> GRGSEDFQYAIDMFKKFIEEAAASMGPEAVKYAKEFLKLLKEYHKNGINNRLLKIALLLLRNQKKIVDKASQDLWRRHPELIAPGGIAFSQRDRALCLRDYGWFLILIVMCLVSGDKGPIEKIGLKCIREMYNSLGVVPAM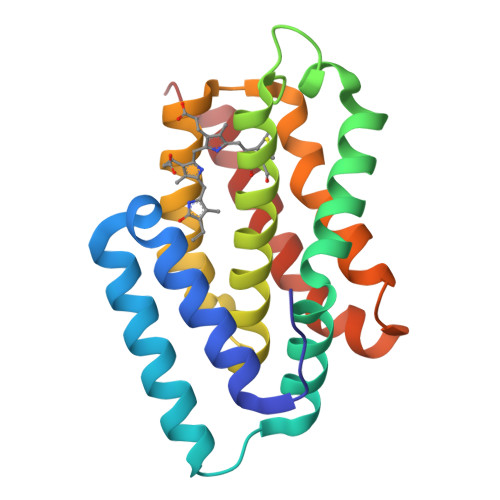MESIRCLKEASLSLLDEEDANETAPYFDYIIKAMSLEHHHHHH> TELKIGNEKVNSTNF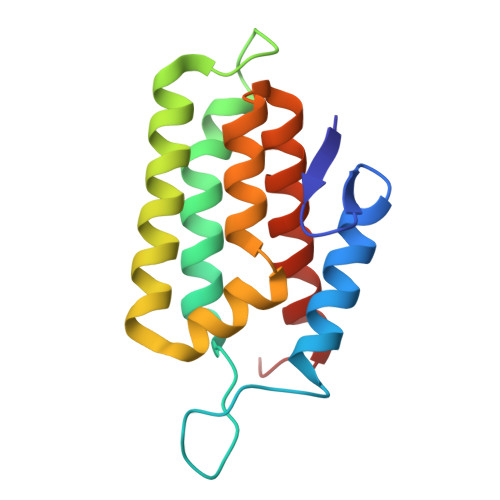GDFAEKAIRGINHKPFVNSKGGEQKITTSKIRGILELVNKVYNRVINTNDVELSENILADIAYIKVKIAYESGREPVVKDFIQRTAFTAAITDVMNQRTRESFLLFARYVESLIAYFKFYGGKD> MATTTPERVMQETMDYHALNAMLNLYDKAGHIQFDKDQQAIDAFFATHVRPHSVTFASQHERLGTLVREGYYDDAVLARYDRAFVLRLFEHAHASGFRFQTFLG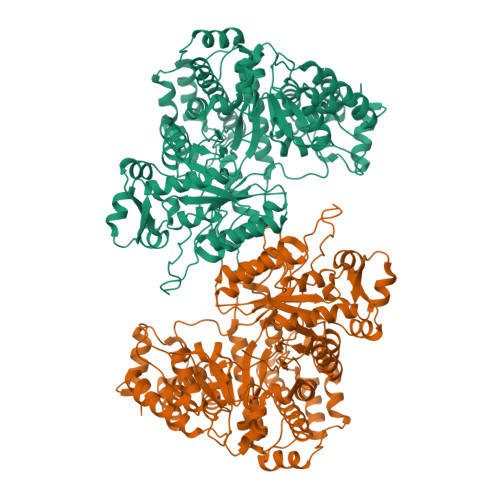AWKFYTSYTLKTFDGKRYLEHFEDRVTMVALTLAQGDETLATQLTDEMLSGRFQPATPTFLNCGKQQRGELVSCFLLRIEDNMESIGRAVNSALQLSKRGGGVAFLLSNLREAGAPIKRIENQSSGVIPVMKMLEDAFSYANQLGARQGAGAVYLHAHHPDILRFLDTKRENADEKIRIKTLSLGVVIPDITFRLAKENAQMALFSPYDIQRRYGKPFGDIAISERYDELIADPHVRKTYINARDFFQTLAEIQFESGYPYIMFEDTVNRANPIAGRINMSNLCSEILQVNSASRYDDNLDYTHIGHDISCNLGSLNIAHVMDSPDIGRTVETAIRGLTAVSDMSHIRSVPSIAAGNAASHAIGLGQMNLHGYLAREGIAYGSPEALDFTNLYFYTITWHAVHTSMRLARERGKTFAGFAQSRYASGDYFTQYLQDDWQPKTAKVRALFARSGITLPTREMWLKLRDDVMRYGIYNQNLQAVPPTGSISYINHATSSIHPIVAKIEIRKEGKTGRVYYPAPFMTNENLDMYQDAYDIGPEKIIDTYAEATRHVDQGLSLTLFFPDTATTRDINKAQIYAWRKGIKSLYYIRLRQLALEGTEIEGCVSCAL>MSAQINNIRPEFDREIVDIVDYVMNYEISSKVAYDTAHYCLLDTLGCGLEALEYPACKKLLGPIVPGTVVPNGVRVPGTQFQLDPVQAAFNIGAMIRWLDFNDTWLAAEWGHPSDNLGGILATADWLSRNAVASGKAPLTMKQVLTAMIKAHEIQGCIALENSFNRVGLDHVLLVKVASTAVVAEMLGLTREEILNAVSLAWVDGQSLRTYRHAPNTGTRKSWAAGDATSRAVRLALMAKTGEMGYPSALTAPVWGFYDVSFKGESFRFQRPYGSYVMENVLFKISFPAEFHSQTAVEAAMTLYEQMQAAGKTAADIEKVTIRTHEACIRIIDKKGPLNNPADRDHCIQYMVAIPLLFGRLTAADYEDNVAQDKRIDALREKIN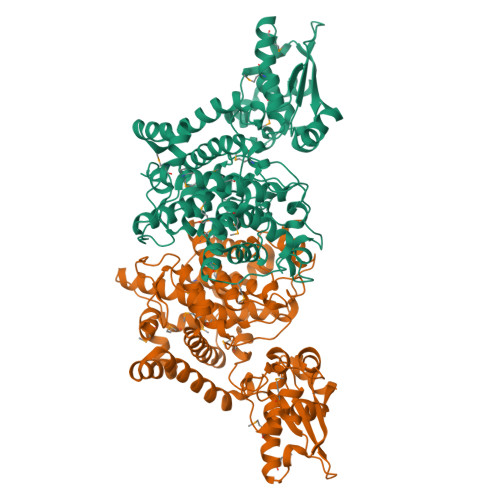CFEDPAFTADYHDPEKRAIANAITLEFTDGTRFEEVVVEYPIGHARRRQDGIPKLVDKFKINLARQFPTRQQQRILEVSLDRARLEQMPVNEYLDLYVI[2x]> MPHVENASETYIPGRLDGKVALVTGSGRGIGA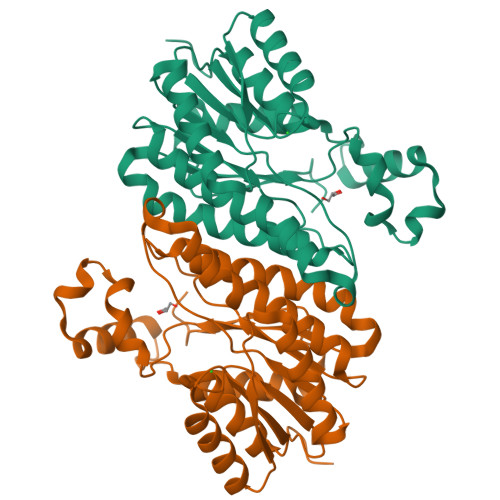AVAVHLGRLGAKVVVNYANSTKDAEKVVSEIKALGSDAIAIKADIRQVPEIVKLFDQAVAHFGHLDIAVSNSGVVSFGHLKDVTEEEFDRVFSLNTRGQFFVAREAYRHLTEGGRIVLTSSNTSKDFSVPKHSLFSGSKGAVDSFVRIFSKDCGDKKITVNAVAPGGTVTDMFHEVSHHYIPNGTSYTAEQRQQMAAHASPLHRNGWPQDVANVVGFLVSKEGEWVNGKVLTLDGGAA> MLVSYLRLQADRRTRHHMMVDGQINPREWFNWHPKEYQPWYFDRHKFLYEQRQYAQFHHLLCHQVYLKDMLHLMR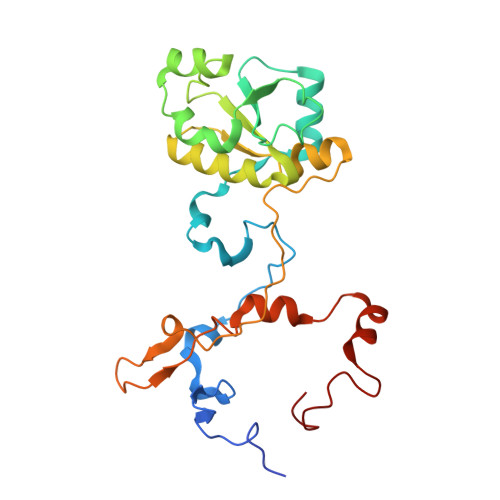YPEPYTHIIDCRTSTQKMHRWVPHSLWLPRDEVEYALQLSADEFLDMYGFRKPDKSDDVILLSHNGIYSEQAGWEWKKQFFQHVYNYRGGTNELFGESYSDMNVSDVLSPWKGPFPQSGVFVDKWSKRKVLTRTGPFDRQYEMQDFALPDLELEKARHPEEGPRQNMPFGLQ>STIT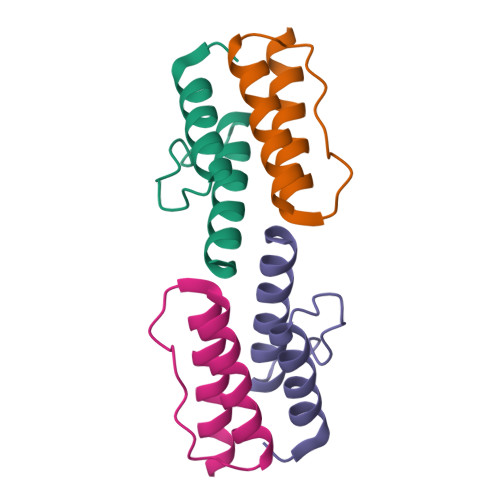RPIIELSNTFDKIAEGNLEAEVPHQNRADEIGILAKSIERLRRSLKVAME[2x]> GCDLERYPLTDLSEETFWNSESNAELALTSLYRGSLTDGVEYNPSDWWSYHGMIMMEHLSDNAFDRRGENNPFFKISSGNLTADNAFIKRYWETSYKRIGYCNRFLVGIQNSSESEKKTRMIAEARFLRATQYFYLASYFKNVPLVENVLTGEEANNVTKTSQADILKWCVTEFTAAAADLPRFSAIPAGEAGRACKQAALAFLGRTCMLQKDWKSGAKAFHDIMELGDNAINANYQELFYPSTGTSNKENIFYIQYLENYLGTGLPQHALSAKDGGWSLVNPAADLYESYEFKDGTPFSYDDPRYDPSNLGKDRDPRLDYTIYYNGAIFMGTEYKMSPDYSAAKKEKLDYTSEASRTGFMMRKYFEESTPINDVQSANGLTPVIRYAEVLLGYLECLVEDNQTITQGILDETINAVRGRASVNMPPVTEVTPAKLREIVRHERRIELAMEGIRYWDIMRWGIAHEVLSQKIWGAPYPGSTQYATTTKEVDPTGNYRWYVGKRAFRNPTDYTWPIPQSEQ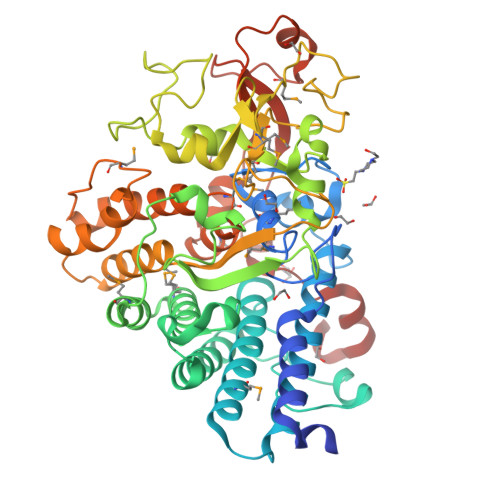NINPNLRD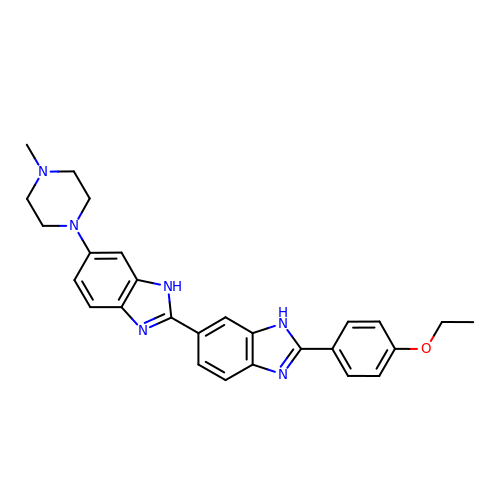2'-(4-ETHOXYPHENYL)-5-(4-METHYL-1-PIPERAZINYL)-2,5'-BI-BENZIMIDAZOLE | C27 H28 N6 O | PRDFBSVERLRRMY-UHFFFAOYSA-N methyl thiophene-2-carboxylate | C6 H6 O2 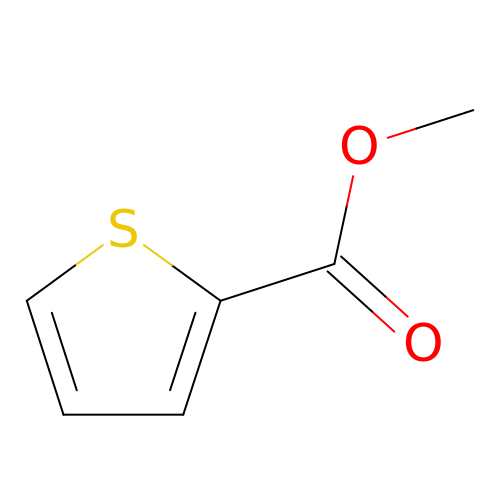S | PGBFYLVIMDQYMS-UHFFFAOYSA-N> ACC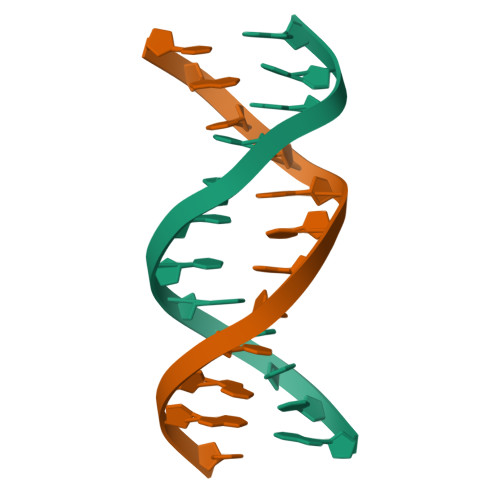GGCGCCACA;> TGTGGCGCCGGT> SMNNKEVELYGGAITTVVPPGFIDASTLREVPDTQEVYVNSRRDEEEFEDGLATNESIIVDLLETVDKSDLKEAWQFHVED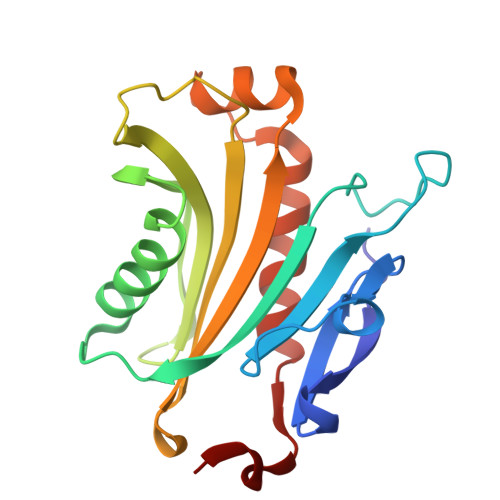LTELNGTTKWEALQEDTVQQGTKFTGLVMEVANKWGKPDLAQTVVIGVALIRLTQFDTDVVISINVPLTKEEASQASNKELPARCHAVYQLLQEMVRKFHVVDTSLFA>SLNE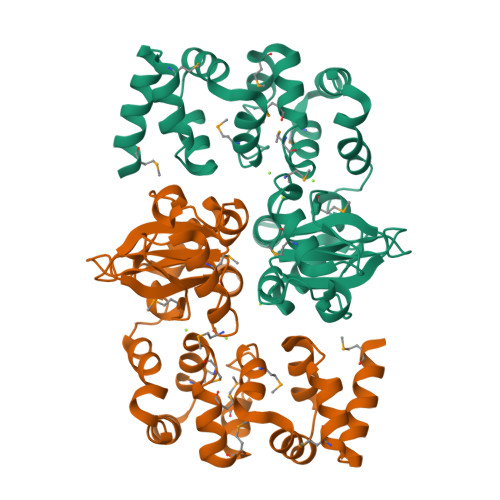GQEMEEQFALLLETLKNQQMNEFRELFLALHIYEQGQFYQSLDEKDRQHLYNYLSPKELADMFDVIEEDNENMKDYLAEMRPSYAADMLAEMYTDNAVDLLNMLDKSQKAKYLSLLSSEEAGEIKELLHYEDETAGAIMTTEFVSIVANQTVRSAMYVLKNQADMAETIYYVYVVDQENHLVGVISLRDLIVNDDDTLIADILNERVISVHVGDDQEDVAQTIRDYDFLAVPVTDYDDHLLGIVTVDDIIDVIDDEAASDYSGLAGVDVEEVSENPLKAASK[2x]>[6x]MFEIKKICCIGAGYVGGPTCSVIAHMCPEIRVTVVDVNESRINAWNSPTLPIYEPGLKEVVESCRGKNLFFSTNIDDAIKEADLVFISVNTPTKTYGMGKGRAADLKYIEACARRIVQN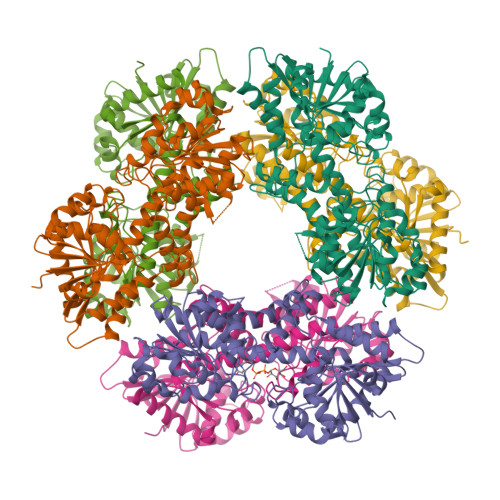SNGYKIVTEKSTVPVRMAESIRRIFDANTKPNLNLQVLSNPEFLAEGTAIKDLKNPDRVLIGGDETPEGQRAVQALCAVYEHWVPREKILTTNTWSSELSKLAANAFLAQRISSINSISALCEATGADVEEVATAIGMDQRIGNKFLKASVGFGGSCFQKDVLNLVYLCEALNLPEVARYWQQVIDMNDYQRRRFASRIIDSLFNTVTDKKIAILGFAFKKDTGDTRESSSIYISKYLMDEGAHLHIYDPKVPREQIVVDLSHPGVSEDDQVSRLVTISKDPYEACDGAHAVVICTEWDMFKELDYERIHKKMLKPAFIFDGRRVLDGLHNELQTIGFQIETIGKKVSSKRIPYAPSGEIPKFSLQDPPNKKPKV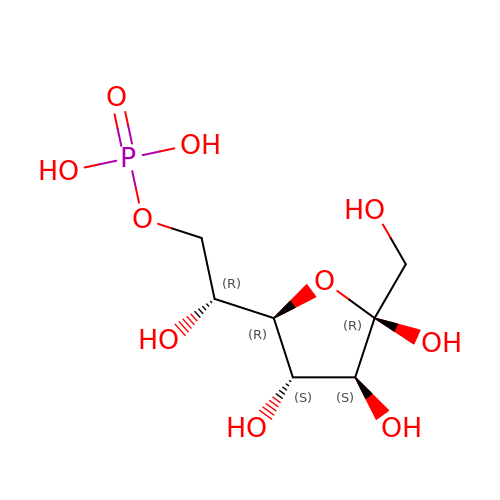1-C-(hydroxymethyl)-6-O-phosphono-beta-D-altrofuranose | C7 H15 O10 P | RKCHIPUTSFLEHR-BNWJMWRWSA-N2,4-bis[(1R)-1-oxidanylethyl]benzene-1,3,5-triol | C10 H14 O5 | 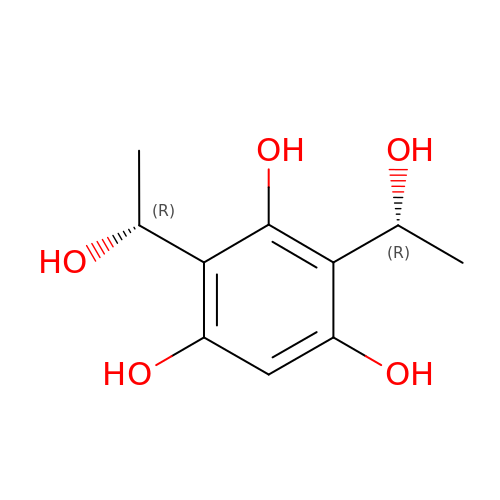HTMUMTIHRQAXFS-RFZPGFLSSA-N>[5x]GSVYPKELTQVFEHYINNNLFDIDSLVKFIEELGYNLEDLATLCLAHLLGYKKLEEPLKREDFLSTWFMQGCSTISDMQECIKTLDVKLHEDLQYFTQIYNYAFNLILDPNRKDIDTDEGIQYWKLFFQPEYPVRMEPDLLEAWFRFLRDEGKTTISKDTWRMLLLFFKRYPTIQKIISDYDETAAWPFIIDEFYECLQDQQ;>GSELNTERQIFLEACIVRIMKAKRNLPHTTLVNEC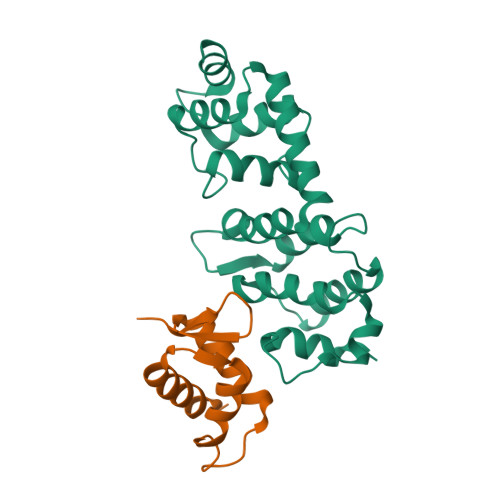IAQSHQRFNAKVSMVKRAIDSLIQKGYLQRGDDGESYAYLA[5x]> ELICIVQRVNESFSLHSGFGGNVYSMKTEPMTGFTNVTKGASVINQKDWIGFGDSRTDLTNDQFPASSDVPLAVAKKFRSLSGASLMLSAFGPPGKVDYLYQGCGKEKVFYEGVNWSPEAGIDCFGSNWTQTKKDFYSRIYEAARSSTCMTLVNSLDTKISSTTATAGTASSCSSSWMKSPLWYAESSVNPGAKPQVCGTEQSATFTLPTSFGIYKCNKHVVQLCYFVYENKAKFNTFGCGDYYQNYYDGNGNLIGGMDNRVAAYRGIANAGVKIECPSKILNPGTYSIKSTPRFLLVPKRSYCFDTDGGYPIQVVQSEWSASRRSDNATEEACLQTEGCIFIKKTTPYVGEADDNHGDIEMRQLLSGLGNN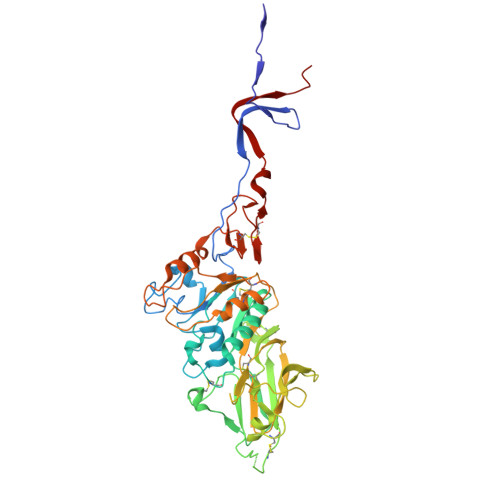DTVCVSQSGYTKGETPFVKDYLSPPKYGRCQLKTDSGRIPTLPSGLIIPQAGTDS> GAMGSLIRKKAAGLESAATIRTKVFVWGLNDKDQLGGLKGSKIKVPSFSETLSALNVVQVAGGSKSLFAVTVEGKVYACGEATNGRLGLGISSGTVPIPRQITALSSYVVKKVAVHSGGRHATALTVDGKVFSWGEGDDGK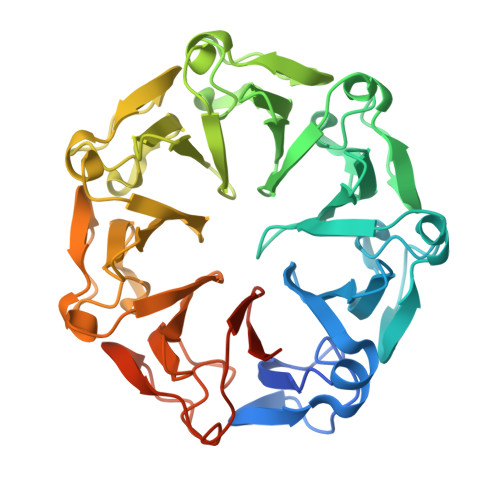LGHFSRMNCDKPRLIEALKTKRIRDIACGSSHSAALTSSGELYTWGLGEYGRLGHGDNTTQLKPKMVKVLLGHRVIQVACGSRDAQTLALTDEGLVFSWGDGDFGKLGRGGSEGCNIPQNIERLNGQGVCQIECGAQFSLALTKSGVVWTWGKGDYFRLGHGSDVHVRKPQVVEGLRGKKIVHVAVGALHCLAVTDSGQVYAWGDNDHGQQGNGTTTVNRKPTLVQGLEGQKITRVACGSSHSVAWTTVDVATPSVHEPVLFQT>MARSRGERTPAARRITSRNARFQQWQALLGNRNKRTRAGEFLVMGVRPISLAVEHGWPVRTLLYDGQRELSKWARELLRTVRTEQIAMAPDLLMELGEKNEAPPEVVAVVEMPADDLDRIPVREDFLGVLFDRPTSPGNIGSIIRSADALGAHGLIVAGHAADVYDPKSVRSSTGSLFSLPAVRVPSPGEVMDWVEARRAAGTPIVLVGTDEHGDCDVFDFDFTQPTLLLIGNETAGLSNAWRTLCDYTVSIPMAGSASSLNAANAATAILYEAVRQRISGRTATTP[2x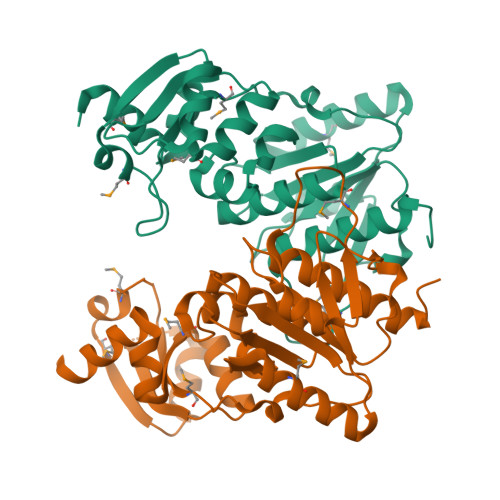]> MAQFAFESDLHSLLQLDAPIPNAPPARWQRKAKEAAGPAPSPMRAANRSHSAGRTPGRTPGKSSSKVQTTPSKPGGDRYIPHRSAAQMEVASFLLSKENQPENSQTPTKKEHQKAWALNLNGFDVEEAKILRLSGKPQNAPEGYQNRLKVLYSQKATPGSSRKTCRYI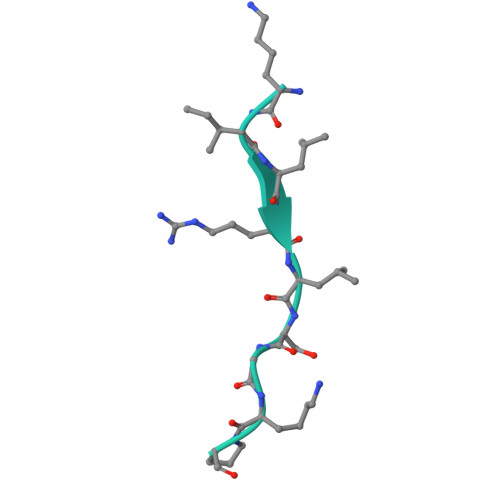PSLPDRILDAPEIRNDYYLNLVDWSSGNVLAVALDNSVYLWSASSGDILQLLQMEQPGEYISSVAWIKEGNYLAVGTSSAEVQLWDVQQQKRLRNMTSHSARVGSLSWNSYILSSGSRSGHIHHHDVRVAEHHVATLSGHSQEVCGLRWAPDGRHLASGGNDNLVNVWPSAPGEGGWVPLQTFTQHQGAVKAVAWCPWQSNVLATGGGTSDRHIRIWNVCSGACLSAVDAHSQVCSILWSPHYKELISGHGFAQNQLVIWKYPTMAKVAELKGHTSRVLSLTMSPDGATVASAAADETLRLWRCFELDPARRREREKASAAKSSLIHQGIR> GSAMGQNPWATTTAFADFMKRFNIPQVHGSGIFVDLGRDTEGYREVGGKCPVFGKAIQMHQPAEYSNNFLDDAPTSNDASKKPLPGGFNNPQVYTSGQKFSPIDDSLLQERLGTAGPKTAIGRCALYAYSTIAVNPSTNYTSTYKYPFVYDAVSRKCYVLSVSAQLLKGEKYCSVNGTPSGLTWACFEPVKEKSSARALVYGSAFVAEGNPDAWQSACPNDAVKDALFGKWEDGQCVPFDTKTSV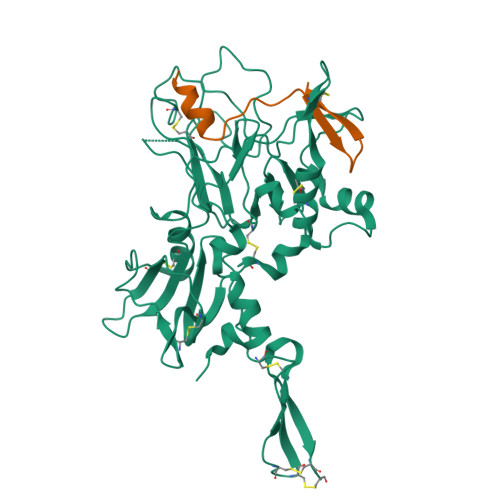QSDQATNKEECWKRVFANPLVASDAPTTYPEAAQKNWNDFWPVHEQSSPKSGGFGANWANFYLEKESGETICAIFDQVPDCFAPITGAVAYTALGSSTEVNLPQCDSASFIPIEGPCNNCVQVVTECVGNQFDQTSKACCTEPEAAALVPR;> GSASDIAQFLTDSGMKAIEDCSWNPIMQQMACVVVAGSGS>MKLQVAIDLLSTEAALELAGKVAEYVDIIELGTPLIKAEGLSVITAVKKAHPDKIVFADMKTMDAGELEADIAFKAGADLVTVLGSADDSTIAGAVKAAQAHNKGVVVDLIGIEDKATRAQEVRALGAKFVEMHAGLDEQAKPGFDLNGLLAAGEKARVPFSVAGGVKVATIPAVQK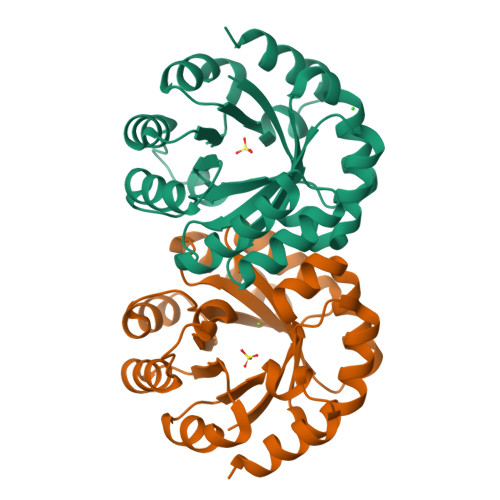AGAEVAVAGGAIYGAADPAAAAKELRAAIA[4x]Cobamides (Cbas) are coenzymes used by cells across all domains of life, but de novo synthesis is only found in some bacteria and archaea. Base activation is catalyzed by a phosphoribosyltransferase (PRTase). To gain insights into the mechanism of base activation by the PRTase from Methanocaldococcus jannaschii (MjCobT), we solved crystal structures of the enzyme in complex with substrate and products. The protein fold consists of an eight-stranded mostly parallel β-sheet with connecting α-helices on both sides where the substrate binding pocket is built from the connecting loops and resides at the end of the C-terminal end of β-strands.

None of the structures described here contain a free base, although they were present in all crystallization experiments. This is true for the apo structure, which contains no ligands in the active site. Superposition of these two structures shows that significant changes occur in the loops extending from Ile 37 to Ile 45, Ser 293 to Lys 314, and Pro 333 to Tyr 348, such that the active site of the apo structure is open to solvent in contrast to that of the complex with either NaMN or α-RP and nicotinic acid. The rms difference between these two structures is 0.94 Å for 329 equivalent residues, indicating the significant conformational changes that occur when substrates bind. Strikingly, residues Lys 173 to Asn 181 that were disordered in the apo structure became ordered upon ligand binding and contribute to the distal component of the binding pocket for the nitrogenous base. Altogether, the movement of the surface loops serves to close the active site on substrate binding.

> MSIIAINENGFLDKIKGRNPLFTCVISSIETTLSIPISGVHRDVIKYTPSADVELVFYGKSLTLKTPPIDATGSPTPATITRACVELKNIKNLHIDAGAFVKPKIPFIEIDEKPTGRIEEGKAMNNSKELYMKGYLLGKNLDAELLIVGESVPGGTTTALGVLLGLGYDAEGKVSSGSINNPHELKIKVVREGLKKAGINEKSSVFDVLNAVGDKMMPVVAGLAISFAERNKPVILAGGTQMSAVLAVIKEINKKVLDKNLIAIGTTEFVLNDKKGDLKGIVEQIGNVPVLASKFYFEKAKIEGLKNYCKGSVKEGVGAGGIAVYSIVNDLEPTKIREFIENKFYEWYKE The activity of GlcNAc transferase V (MGAT5) primes the biosynthesis of an N-glycan antenna that is heavily upregulated in cancer. Introduction of this 6-linked GlcNAc residue is mediated by the enzyme MGAT5, and ensuing elongation by other GTs can give rise to a long glycan chain that serves as a ligand to immunomodulatory galectins. Overexpression of MGAT5 is frequently observed in a range of malignant tumors and generally associated with a worse prognosis. MGAT5 transfers GlcNAc to the NGA2 N-glycan intermediate in the secretory pathway. Here, we report the development of a BH strategy for MGAT5 as a GlcNAc transferase with outstanding biological relevance.

Toward capturing a BH-MGAT5/UDP-GlcNButAz 6/M592 crystal complex, we crystallized a variant of BH-MGAT5 bearing a substitution of the catalytic Glu297 to Ala to prevent UDP-GlcNButAz 6 turnover without altering the fold of the enzyme. However, soaking experiments using UDP-GlcNButAz 6 ± M592 failed to yield any structures of the binary or ternary complexes. To understand how the BH mutations are positioned within the active site, we solved a crystal structure of the triple MGAT5 variant E297A/F458V/F517L in complex with UDP and M592. This structure closely aligned with the corresponding WT-MGAT5 ternary complex, with a root-mean-square deviation of 0.49 Å over the entire protein (988 aligned residues for chains A and B, superposed by Cα atoms). The gatekeeper residues in WT-MGAT5, Phe458 and Phe517 overlaid directly with the BH-MGAT5 variant residues, Val458 and Leu517 (insert). While the latter amino acid side chains adopted a similar spatial trajectory as the parental Phe side chains, the space occupied is substantially smaller, enlarging the active site as a defining feature of BH engineering. We further investigated the combination of UDP-GlcNButAz 6 with MGAT5F458V/F517L, now called BH-MGAT5, that showed the most favorable conversion among all putative BH-enzyme/substrate pairs. We found that the azide group is preferentially oriented toward F458V and F517L, well positioned in the cavity created by the BH substitutions. In contrast, our BH-MGAT5 variant displayed increased acceptance of UDP-GlcNButAz 6 while completely losing activity against UDP-GlcNAc 1. Taken together, BH-MGAT5/UDP-GlcNButAz 6 are a selective enzyme–substrate pair, mainly driven by the negligible activity of BH-MGAT5 toward UDP-GlcNAc 1 compared to WT-MGAT5.

>[2x]SLAEIRTDFNILYSMMKKHEEFRWMRLRIRRMADAWIQAIKSLAEKQNLEKRKRKKVLVHLGLLTKESGFKIAETAFSGGPLGALVQWSDLITSLYLLGHDIRISASLAELKEIMGGGGVELIYIDIVGLAQFKKTLGPSWVHYQCMLRVLDSFGTEPEFNHANYAQSKGHKTPWGKWNLNPQQFYTMFPHTPDNSFLGFVVEQHLNSSDIHHINEIKRQNQSLVYGKVDSVWKNKKIYLDIIHTYMEVHATVYGSSTKNIPSYVKNHGILSGRDLQFLLRETKLFVGLGLPYEGPAPLEAIANGCAFLNPKFNPPKSSKNTDFFIGKPTLRELTSQHPYAEVFIGRPHVWTVDLNNQEEVEDAVKAILNQKIEPYMPYEFTCEGMLQRINAFIEKQDFCHGQVMWPPLSALQVKLAEPGQSCKQVCQESQLICEPSFFQHLNKDKDMLKYKVTCQSSELAKDILVPSFDPKNKHCVFQGDLLLFSCAGAHPRHQRVCPCRDFIKGQVALCKDCL> MGSSHHHHHHSSGRENLYFQGDIPQQLVERLQEEKRIEAQKRKERQEAHLYMQVQIVAEDQFCGHQGNDMYDEEKVKYTVFKVLKNSS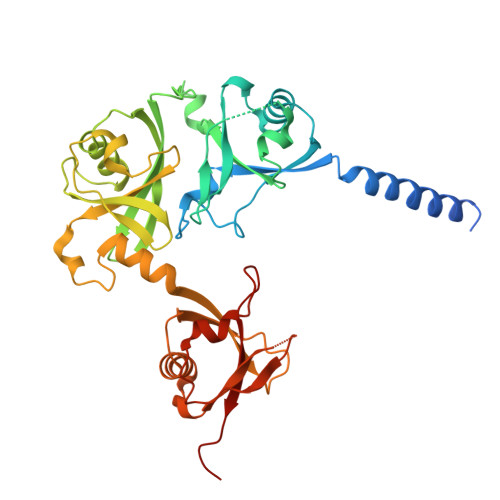LAEFVQSLSQTMGFPQDQIRLWPMQARSNGTKRPAMLDNEADGNKTMIELSDNENPWTIFLETVDPELAASGATLPKFDKDHDVMLFLKMYDPKTRSLNYCGHIYTPISCKIRDLLPVMCDRAGFIQDTSLILYEEVKPNLTERIQDYDVSLDKALDELMDGDIIVFQKDDPENDNSELPTAKEYFRDLYHRVDVIFCDKTIPNDPGFVVTLSNRMNYFQVAKTVAQRLNTDPMLLQFFKSQGYRDGPGNPLRHNYEGTLRDLLQFFKPRQPKKLYYQQLKMKITDF> AEFDRITNFGDALSDIGNKHMITVDMNQATSGKIGIRADKPNFDGRFSNGPVWTEYL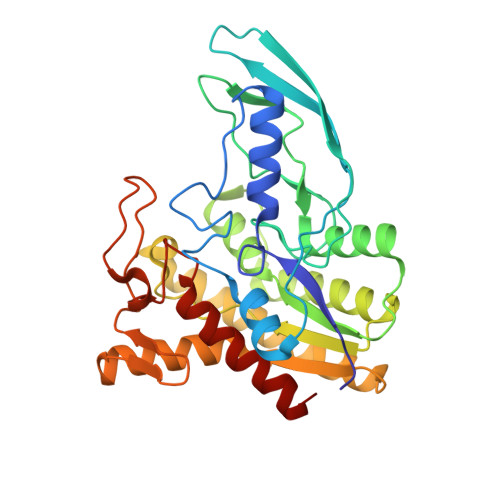AGFLAKPAPVRGHGEIDSQVVLKDQAGKQITYHYHHNALPGTNWAVGGAMSGLGNFLDIDAANGFTAKSGLDVLTNTGQQIKLRIANKGQFTGNELVSYMSGTNNLWFTLFGDLDQTGNKAAGFALTDIETLIDAGAKQVLAANIPDFVDAPWFAGQQKKTTRFIQSHNQALKAGLDQLAAAHPDVEIYYFDAFDLFNKVSNEVKTKGKYQDKELAITLTNVTGEAYSYATGKVIAQPNRNLFWDGLHPTTAMHKIMAKEAASLVISGRTL> MVRFKHRYLLCELVSDDPRCRLSLDDRVLSSLVRDTIARVHGTFGAAACSIGFAVRYLNAYTGIVLLRCRKEFYQLVWSALPFITYLENKGHRYPCFFNTLHVGGTIRTCQKFLIQYNRRQLLILLQNCTDEGEREAIQKSVTRSCLL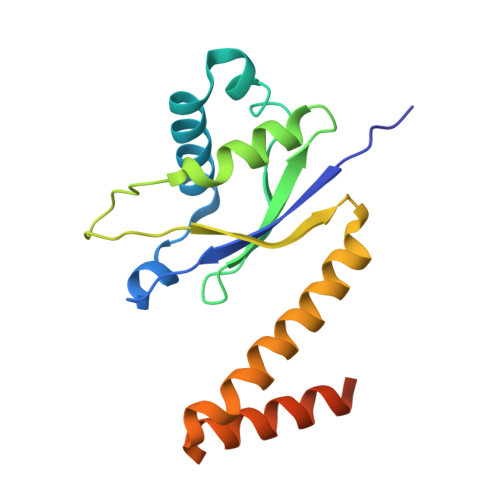EEEEESGEEAAEAME> GG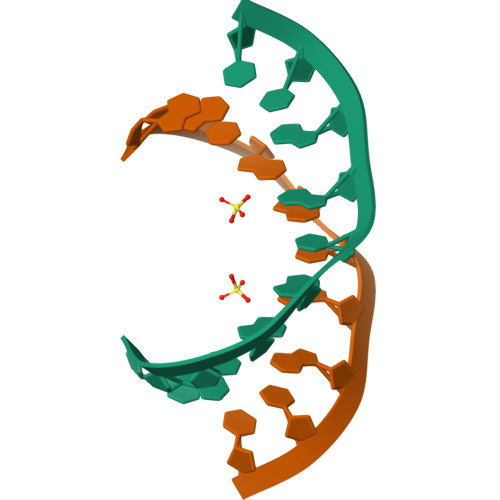CAGCAGCC>[2x]MPYIVDVYAREVLDSRGNPTVEVEVYTETGAFGRALVPSGASTGEYEAVELRDGDKDRYLGKGVLTAVNNVNEIIAPELLGFDVTEQNAIDQLLIELDGTENKGKLGANAILGVSMACARAAADFLQIPLYQYLGGFNSKTLPVPMMNIVNGGEHADNNVDIQEFMIMPVGAPNFREALRMGAQIFHSLKSVLSAKGLNTAVGDEGGFAPNLGSNEEALQTIVEAIEKAGFKPGEEVKLAMDAASSEFYNKEDGKYHLSGEGVVKTSAEMVDWYEELVSKYPIISIEDGLDENDWEGHKLLTERLGKKVQLVGDDLFVTNTKKLSEGIKNGVGNSILIKVNQIGTLTETFDAIEMAKRAGYTAVISHRSGETEDSTIADIAVATNAGQIKTGAPSRTDRVAKYN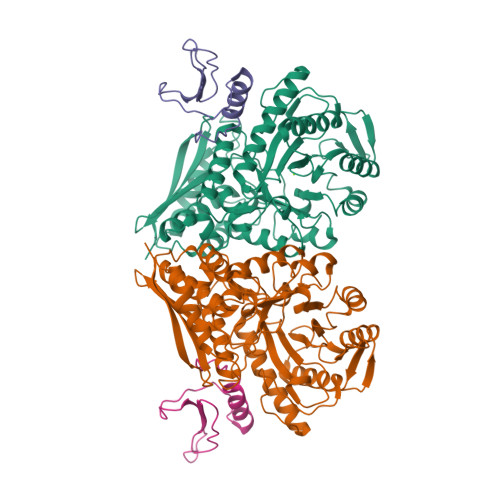QLLRIEDQLAETAQYHGINSFYNLNK;>MLNQVEVLREEYVEGYVVQMWRRNPSNAPVIEVFTEDNLEEGIIPEYVTANDDTFDRIVDAVEFGYLEELELV[2x]>MKMPAYEFWFVVGSQHLYGDEALAQVEAHAREMVPALQAAVGNAHVLRWKGVLKDADEIRRLCLEASADDVCAGVIAWMHTFSPAKMWIRGLLALRKPLLHLHTQFN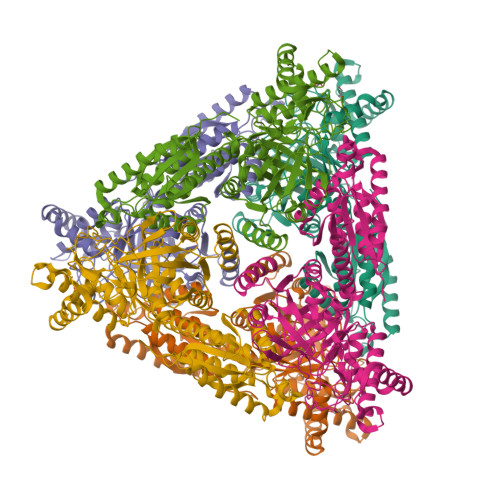RDIPWDTIDMDFMNLNQSAHGDREYGFIGARMGVARKVVVGHWEDPEVRERLAKWMRTAVAFAESRNLKVARFGDNMREVAVTEGDKVGAQIQFGWSVNGYGIGDLVQYIRDVSEQKVNELLDEYEELYDIVPAGRQEGPVRESIREQARIELGLKAFLQDGNFTAFTTTFEDLHGLKQLPGLAVQRLMQQGYGFAGEGDWKTAALLRIMKVMSTGLQGGTSFMEDYTYHFEKGNDLVLGSHMLEVCPSIAAEEKPILDVQHLGIGGKDDPARLVFDGGEGAAVNASLIDLGHRFRLIVNEVDAVKPEHDMPKLPVARILWKPRPSLRDSAEAWILAGGAHHTCFSFAVTTEQLQDFAEMAGIECVVINEHTSVSSFKNELKWNEVFWRGR[6x]> MPRPRVLLLGDPARHLDDLWSDFQQKFEVIPANLTTHDGFKQALREKRYGDFEAIIKLAVENGTESYPWNADLISHLPSSLKVFAAAGAGFDWLDLDALNERGVAFANSRGAGDT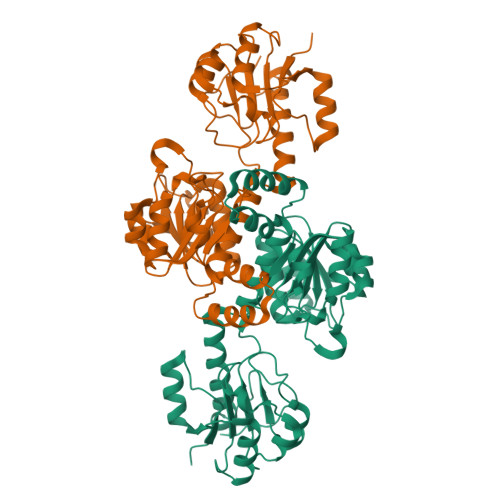ATSDLALYLILSVFRLASYSERAARTGDPETFNRVHLEIGKSAHNPRGHVLGAVGLGAIQKEIARKAVHGLGMKLVYYDVAPADAETEKALGAERVDSLEELARRSDCVSVSVPYMKLTHHLIDEAFFAAMKPGSRIVNTARGPVISQDALIAALKSGKLLSAGLDVHEFEPQVSKELIEMKHVTLTTHIGGVAIETFHEFERLTMTNIDRFLLQGKPLLTPAGKVFAPSSAA;> MPRPRVLLLGDPARHLDDLWSDFQQKFEVIPANLTTHDGFKQALREKRYGDFEAIIKLAVENGTESYPWNADLISHLPSSLKVFAAAGAGFDWLDLDALNERGVAFANSRGAGDTATSDLALYLILSVFRLASYSERAARTGDPETFNRVHLEIGKSAHNPRGHVLGAVGLGAIQKEIARKAVHGLGMKLVYYDVAPADAETEKALGAERVDSLEELARRSDCVSVSVPYMKLTHHLIDEAFFAAMKPGSRIVNTARGPVISQDALIAALKSGKLLSAGLDVHEFEPNVSKELIEMKHVTLTTHIGGVAIETFHEFERLTMTNIDRFLLQGKPLLTPAGKVFAPSSAA>PNLTIVVVSELLHTNWTDYVCLLESRFPDLQINIVSAPQEDALQMLLDGSAQLALMFEREHLDNREQFVELKREALIPVISKTHPLASQEHVSYEQILGTRQIVVASRDETLKPELLFSKHYWRTDNHHSACLMILRNLGWGVLPQEMFKENPE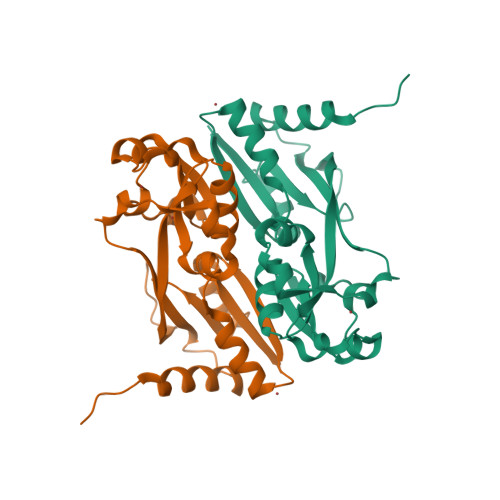LNNKLKALDVFDFTPRFEYYVDLVWSRESELGAAARFLIDYIRNKRMQPAPLEHHHHHH[2x]>[2x]SNAAPQQINDIVHRTITPLIEQQKIPGMAVAVIYQGKPYYFTWGYADIAKKQP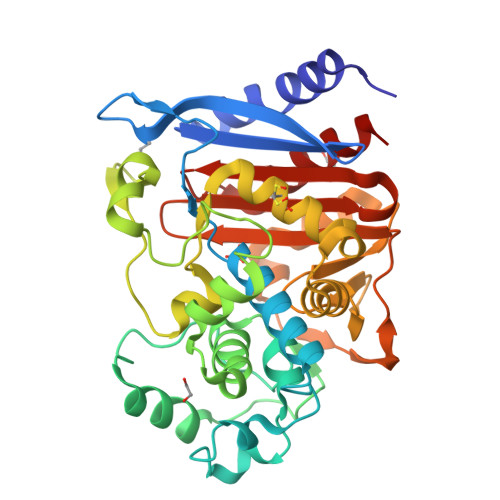VTQQTLFELGSVSKTFTGVLGGDAIARGEIKLSDPATKYWPELTAKQWNGITLLHLATYTAGGLPLQVPDEVKSSSDLLRFYQNWQPAWAPGTQRLYANSSIGLFGALAVKPSGLSFEQAMQTRVFQPLKLNHTWINVPPAEEKNYAWGYREGKAVHVSPGALDAETYGVKSTIEDMACWVRSNMNPRDINDKTLQQGIQLAQSRYWQTGDMYQGLGWEMLDWPVNPDIIVNGSDNKIALAARPVKAITPPTPAVRASWVHKTGATGGFGSYVAFIPEKELGIVMLANKNYPNPARVAAAWQILNALQ N-phenylthioformamide | 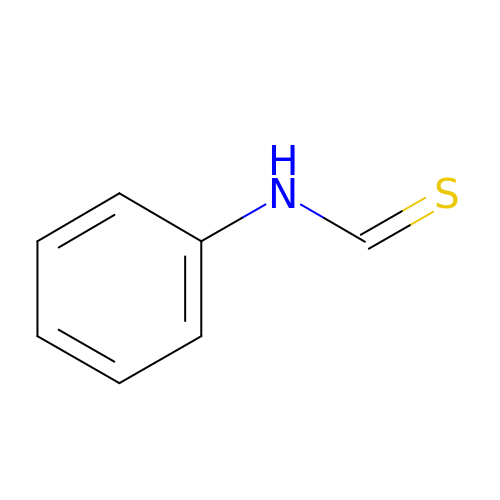C7 H7 N S | UNRRVOATHRPYDX-UHFFFAOYSA-N>[2x]MNAVEIISRDIYKAIDIQTKI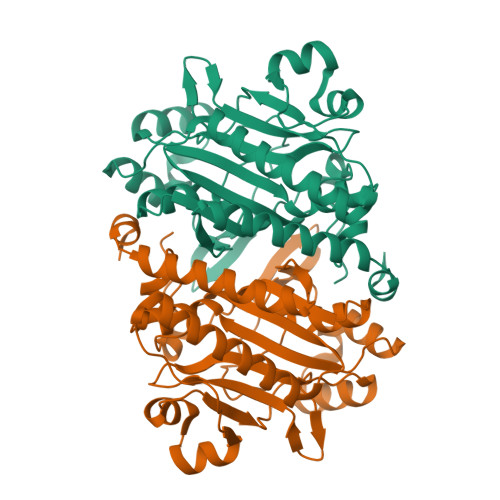LDYMTKFFTDRGFKWLLPIMLSPITDPLWPDPAGEGIRPAEVDVYGVRMRLTHSMILHKQLAIAMGLEKIFVLSPNIRLESRRKDDGRHSYEFTQLDFEIEGAKMKDVMRLIEELIYGLFRKAEEWTGREFPRARHFKVYDYKDILEEFGSDEKASMEMEEPFWIVNIPREFYDREENGVWKNYDLILPYGYGEVSSGGEREWEYEKIVAKIRAAGLKEDSFRPYLEIARAGKLKPSAGAGIGVERLVRFIVGAKHIAEVQPFPRVPGIPAVI5-[[(2~{R})-1-([1,2,4]triazolo[1,5-a]pyrimidin-7-yl)pyrrolidin-2-yl]methoxy]isoquinoline 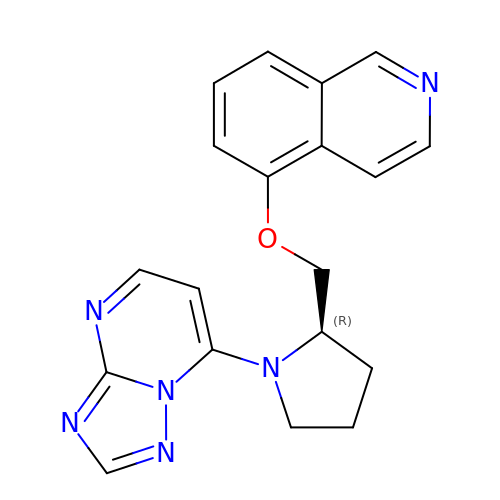| C19 H18 N6 O | UCCCEISNAUTIDA-OAHLLOKOSA-N Human endonuclease VIII-like 1 (hNEIL1) is a bifunctional DNA glycosylase of the Fpg/Nei family, which catalyzes the removal of damaged bases and subsequent incision of the newly generated abasic sites. Unlike traditional enzymes which are commonly referred to as highly specific biocatalysts, one special feature for hNEIL1 is its unique capability to recognize a wide range of substrates, including formamidopyrimidines, hydantoin lesions, oxidized, and dihydro-modified pyrimidine bases, derived from all four canonical bases. Here, by integrating structural, computational, and biochemical investigations, we show that hNEIL1 uses a triage mechanism to achieve broad specificity and reduce futile repair of normal bases. This mechanism involves two mutually competing interaction states: an activated state that commits catalysis and BER, and a quarantine state that temporarily separates and prevents the flipped base from catalysis via auto-inhibition.

While we also crystallized the complex structures for more lesions in this study, we were unable to obtain intact substrates in the active site of hNEIL1, presumably due to the residual glycosylase activity. Hence, we introduced an extra E3Q mutation to the truncated hNEIL1(C∆95 P2G) (see the “Methods” section) and succeeded in the determination of complex structures containing 5-hydroxyuracil (5-OHU), spiroiminodihydantoin 1 (Sp1), (S)-guanidinohydentoin (Gh), dihydrothymine (DHT) and dihydrouracil (DHU), respectively. Despite the very different chemical structures of these substrates, they are recognized similarly by hNEIL1. The damaged bases are fully extruded from the DNA helix and inserted into a relatively loose binding pocket, which allows the accommodation of substrates with varying sizes and shapes. One edge of the flipped base points towards the protein and forms close contact with the side chain of K242. Noteworthy, across all these structures, we observed an unusually short distance (~3.0 Å) between an outwards heterocyclic nitrogen atom of the nucleobases and the terminal nitrogen atom of residue 242. Based on the similar overall conformation and detailed atomic interactions, we conclude that such a tautomerization-dependent mechanism may be a general strategy for hNEIL1 to recognize not only Tg but also 5-OHU, Sp1, Gh, DHT, and DHU. Accordingly, K242 is more likely to retain the base in the activated state compared to R242, or in other words, the activated state is more favored by the genomically encoded hNEIL1(K242) compared to its RNA-edited counterpart, which is supported by our QM/MM calculations.

>[3x]MGQGPELHLASQFVNEACRALVFGGCVEKSSVSRNPEVPFESSAYRISASARGKELRLILSPLPGAQPQQEPLALVFRFGMSGSFQLVPREELPRHAHLRFYTAPPGPRLALCFVDIRRFGRWDLGGKWQPGRGPCVLQEYQQFRENVLRNLADKAFDRPICEALLDQRFFNGIGNYLRAEILYRLKIPPFEKARSVLEALQQHRPSPELTLSQKIRTKLQNPDLLELCHSVPKEVVQLGGKGYGSESGEEDFAAFRAWLRCYGMPGMSSLQDRHGRTIWFQGDPGPLAPKGRKS>[2x]MASSSLLSFSLCLLLLCHLSQAQFGSSQESPFQSPRRSVSSRNECRIERLNAL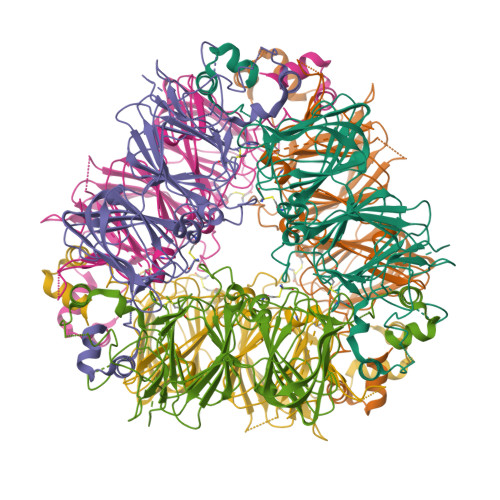EPTRTVRSEAGVTDYFDEDNEQFRCAGVSTIRRVIEPRGLLLPSMSNAPRLVYIVQGRGIVGLVMPGCPETFQSFQRSEREEGERHRWSRDEHQKVYQFQEGDVLAVPNGFAYWCYNNGENPVVAITVLDTSNDANQLDRSHRQFLLAGRQEQGRQRYGREGSIKENILRGFSTELLAAAFGVNMELARKLQCRDDTRGEIVRAENGLQVLRPSGMEEEEREEGRSINGFEETYCSMKIKQNIGDPRRADVFNPRGGRITTLNSEKLPILRFIQMSAERVVLYRNAMVSPHWNINAHSIMYCTGGRGRVEVADDRGETVFDGELRQGQLLIVPQNFAMLERAGSAGFQLVSIKTSDRAMVSTVVGKTSALRGMPVEVLMNSYRLSRDEARRVKLTRGDEVAIFTPRRESRAEA[2-([2-(2-amino-6-oxo-1,6-dihydro-9H-purin-9-yl)ethyl]{2-[(2-oxoethyl)(2-phosphonoethyl)amino]ethyl}amino)ethyl]phosphonic 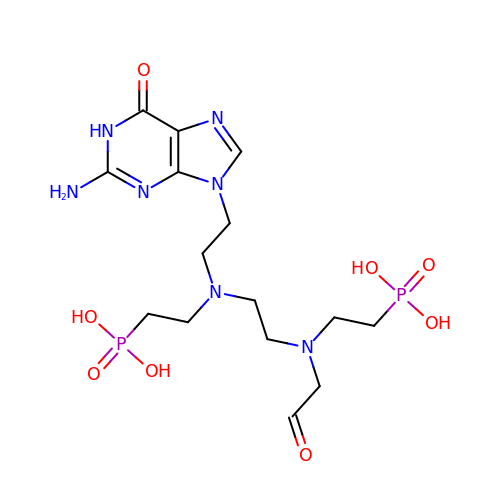acid | C15 H27 N7 O8 P2 | UVQNMNMHDDJCKT-UHFFFAOYSA-N>MLPGTFFEVLKNKGVVAIATQGEDGPHLVNTWNSYLKVLDGNRIVVPVGGMHKTEANVARDERVLMTLGSRKVAGRNGPGTGFLIRGSAAFR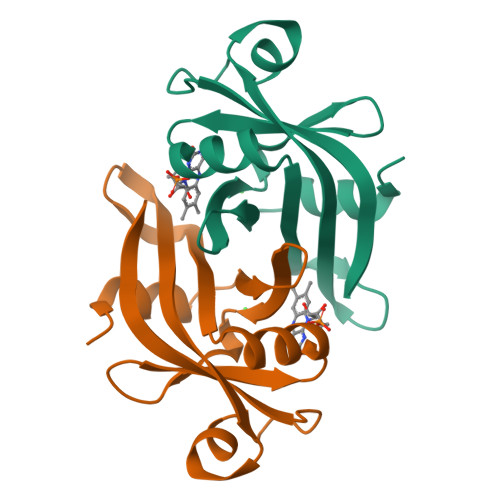TDGPEFEAIARFKWARAALVITVVSAEQTL[2x]>[2x]GMNNSLAFNHDTLPQKVMFGYGKSSAFLKQEVERRGSAKVMVIAGEREMSIAHKVASEIEVAIWHDEVVMHVPIEVAERARAVATD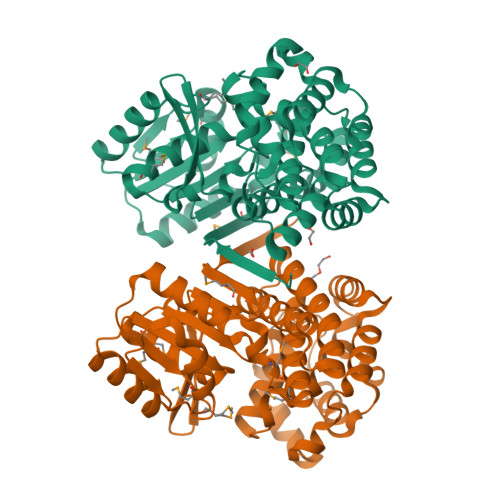NEIDLLVCVGGGSTIGLAKAIAMTTALPIVAIPTTYAGSEATNVWGLTEAARKTTGVDLKVLPETVIYDSELTMSLPVEMSVASGLNGLAHCIDSLWGPNADPINAVLAAEGIRALNQGLPKIVANPHSIEGRDEALYGAYLAAVSFASAGSGLHHKICHTLGGTFNLPHAQTHATVLPYVLAFNAGDAPEAERRAAAAFGTDTALEGLQRLRLSVNAPKRLSDYGFEASGIAEAVDVTLEKVPANNPRPVTRENLSRLLEAALNGEDPAVLSAVLSN>[4x]KDKKTLEEYSGIIYVSRLPHG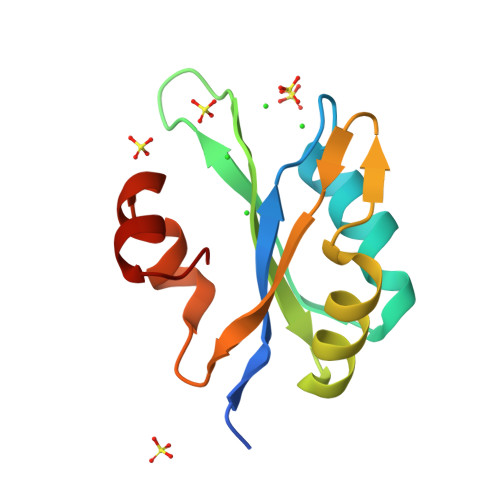FHEKELSKYFAQFGDLKEVRLARNKKTGNSRHYGFLEFVNKEDAMIAQESMNNYLLMGHLLQVRVLPKGAKIEKLYKYKKRVLVEKGITK> AAELIKYNQTGMTLNQVAQIQAGLQYKPQVQRVPGKWTDANFNDVKHAMDTKRLAQDPALKYQFLRLDQPQNISIDKINQFLKGKGVLENQGAAFNKAAQMYGINEVYLISHALLETGNGTSQLAKGADVVNNKVVTNSNTKYHNVFGIAAYDNDPLREGIKYAKQAGWDTVSKAIVGGAKFIGNSYVKAGQNTLYKMRWNPAHPGTHQYATDVDWANIN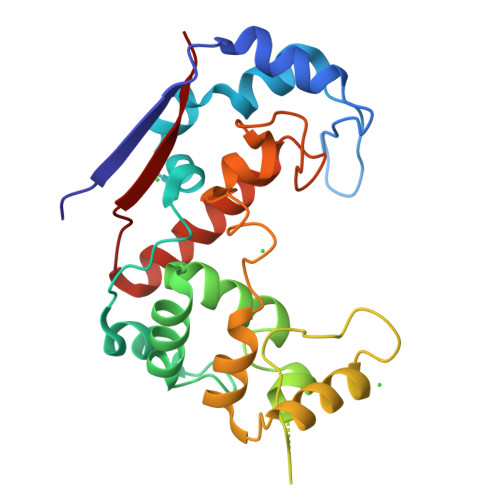AKIIKGYYDKIGEVGKYFDIPQYK> MSAIERITKAAHLIDMNDIIREGNPTLRTVAEEVTFPLSDQEIILGEKMMQFLKHSQDPVMAEKMGLRGGVGLAAPQL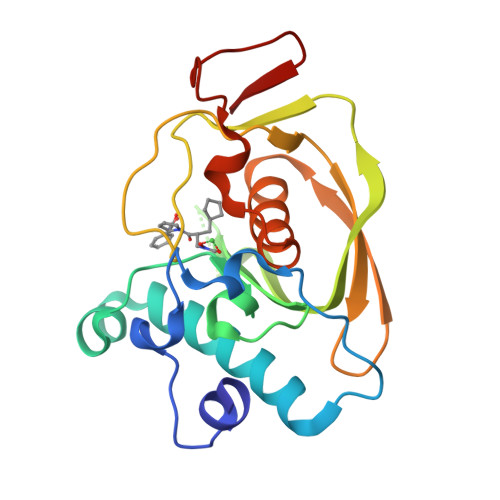DISKRIIAVLVPNIVEEGETPQEAYDLEAIMYNPKIVSHSVQDAALGEGEGCLSVDRNVPGYVVRHARVTVDYFDKDGEKHRIKLKGYNSIVVQHEIDHINGIMFYDRINEKDPFAVKDGLLILE AMMOSAMIDE 272 | C13 H12 N4 O3 | 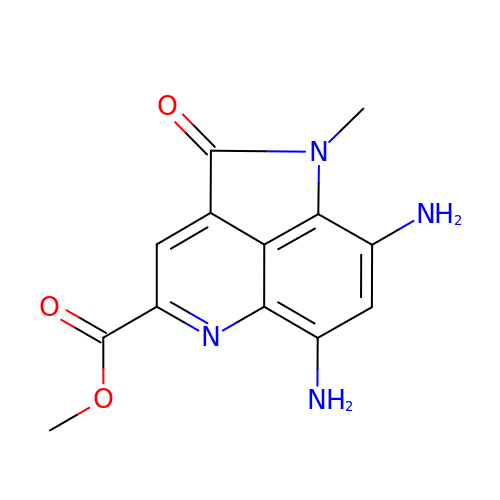LBJXTHMUZLBEBR-UHFFFAOYSA-N>EAEAEFDSNTKGWSEVLKGSECKPRPIVVPVSETHPELTSQRFNPPCVTLMRCGGC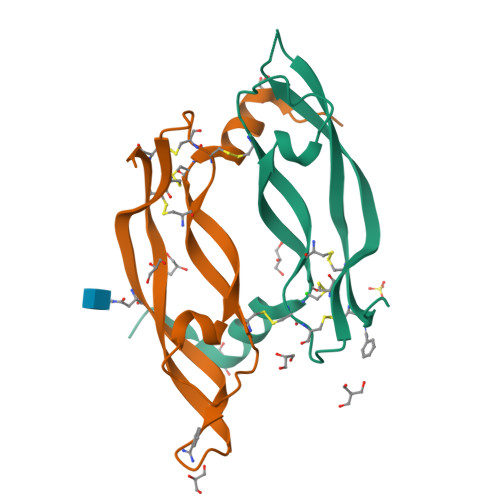CNDESLECVPTEEVNVTMELLGASGSGSNGMQRLSFVEHKKCDCRPRFTTTPPTTTRPPRRRRVDHHHHHH[4x]>[2x]GPGSEDDICILNHEKGSGSSRHSEKIAIRDFQVGDLVLIILDERHDNYVLFTVSPTLYFLHSESLPALDLKPGEGASGASR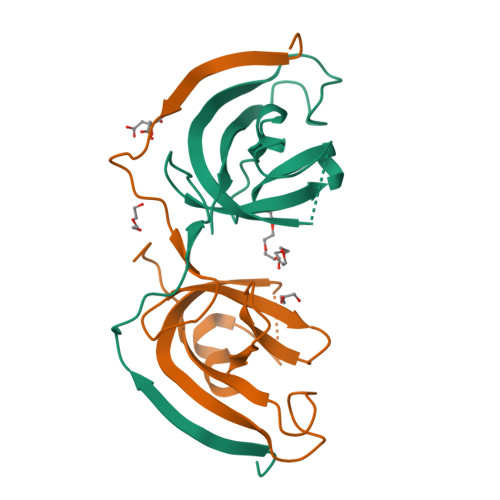RPWVLGKVMEKEYCQAKKAQNRFKVPLGTKFYRVKAVSWNKKV>MDGRGGRSTTEPVTMTLDVKNDQVAKHDFGKPGMDVGDMDIFSDILSVDGKQVGYDGGACFFTNVTPDNPMTYCELTIHLDAGEIFARSLTPHTLAPFTMAITGGTGEYANSKGELTVSGVATPDEKY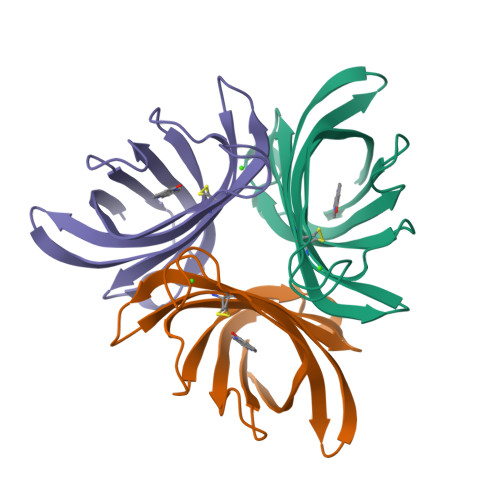ELKLTKAENLYFQ[3x]>MAADAPGDRMEEPLPDRAVPIYVAGFLALYDSGDSGELALDPDTVRAALPPDNPLPINVDHRAGCEVGRVLAVVDDPRGPFFVGLIACVQLERVLETAASAAIFERRGPPLSREERLLYLITNYLPSVSLATKRLGGEAHPDRTLFAHVALCAIGRRLGTIVTYDTGLDAAIAPFRHLSPASREGARRLAAEAEIALSGRTWAPGVEALTHTLLSTAVNNMMLRDRWSLVAERRRQAGIAGHTYLQASEKFKMWGAEPVSAPARGYKNGAPESTDIPPGSIAAAPQGDRCPIVRQRGVALSPVLPPMNPVPTSGTPAPAPPGDGSYLWIPASHYNQLVAGHAAPQPQPHSAFGFPAAAGAVAYGPHGAGLSQHYPPHVAHQYPGVLFSGPSPLEAQIAALVGAIAADRQAGGQPAAGDPGVRGSGKRRRYEAGPSESYCDQDEPDADYPYYPGEARGGPRGVDSRRAARQSPGTNETITALMGAVTSLQQELAHMRARTSAPYGMYTPVAHYRPQVGEPEPTTTHPALCPPEAVYRPPPHSAPYGPPQGPASHAPTPPYAPAACPPGPPPPPCPSTQTRAPLPTEPAFPPAATGSQPEASNAEAGALVNASSAAHVDVDTARAADLFVSQMMGAR[12x];>MTAPRSWAPTTRARGDTEALCSPEDGWVKVHPTPGTMLFREILHGQLGYTEGQGVYNVVRSSEATTRQLQAAIFHALLNATTYRDLEADWLGHVAARGLQPQRLVRRYRNAREADIAGVAERVFDTWRNTLRTTLLDFAHGLVACFAPGGPSGPSSFPKYIDWLTCLGLVPILRKRQEGGVTQGLRAFLKQHPLTRQLATVAEAAERAGPGFFELALAFDSTRVADYDRVYIYYNHRRGDWLVRDPISGQRGECLVLWPPLWTGDRLVFDSPVQRLFPEIVACHSLREHAHVCRLRNTASVKVLLGRKSDSERGVAGAARVVNKVLGEDDETKAGSAASRLVRLIINMKGMRHVGDINDTVR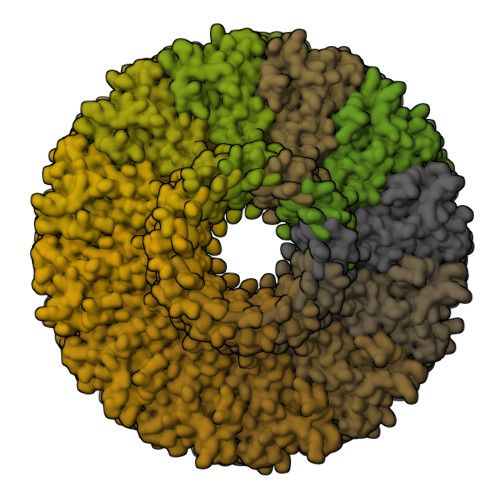AYLDEAGGHLIDAPAVDGTLPGFGKGGNSRGSAGQDQGGRAPQLRQAFRTAVVNNINGVLEGYINNLFGTIERLRETNAGLATQLQERDRELRRATAGALERQQRAADLAAESVTGGCGSRPAGADLLRADYDIIDVSKSMDDDTYVANSFQHPYIPSYAQDLERLSRLWEHELVRCFKILCHRNNQGQETSISYSSGAIAAFVAPYFESVLRAPRVGAPITGSDVILGEEELWDAVFKKTRLQTYLTDIAALFVADVQHAALPPPPSPVGADFRPGASPRGRSRSRSPGRTAPGAPDQGGGIGHRDGRRDGRR[12x]> MLPEFPKIAVVAGSEAESVFRVVDIGTGDVVYEGRLSDSVYDDASGDTVRHADFGEWKRPGSYSVTVGRSSSAPFRIGNDVYRAPLIQAARSYTLARAGVAIDDPVTGLRHDVGHAQDKQAMLFFEDPFHRQGDPIDVSGGWYDAGDYGKYVPTGAVAAAQLMLAWEMRPELWRSLSLSLPAGLSEPERRAGLPDLLVEIKYELDWLLRMQRPDGAVYLKVAGGAWPGYIRPEEDTADRYVFGLSTYGTAQFAGAAAMGARVYAPFLPDYARKLLDAAIRAQRYLEQHPDPEFRYDEGQNNGSGPYEKRTDREERFWAAAELLRTTDDARYDAYIREHFSDFLEGKTSAVFWGNTVLLGQWAYVNAERADADHKASVRASLTAYADELVRWASANGYRSVLRPTDYFWGSAREAMGRAQALLLADAVAPNRAYLETALDQAHWLFGRNAAGTSFMTGIGMHSPQKPHHRLVASTQTLIPGLVVGGPNAQGGDPIMDRLLRESDPRVFPAKAYVDDWEAYSVNEPAIDYTAPAVFVLTRFAED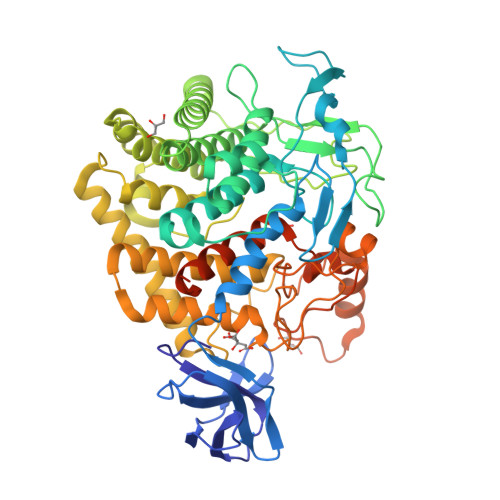RGSGENLYFQGWSHPQFEKNSAVDGSGHHHHHHHH>[2x]MVRQHAGPRDRSEIVTTSTGTNGRHTVAGPGSAGPVGYSLPLSPTGESAMLTPPPWHFSGEVVMVDYRVDPDAARRFLPPGLEPGADPGA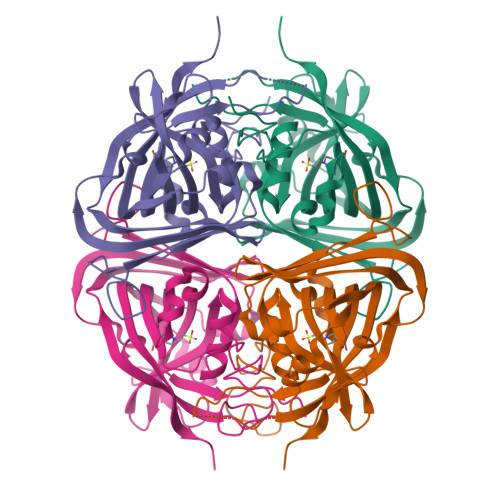AAAVFATWQWCSQDGAELTDPGRCQFGEFLILLSCEFEGRPMARCPYAWVDQAVPMMRGWVQGMPKQFGVIHQSRPVTVGKAGSRLAPGGRFDGALSVHGRRVVEASVTVDRSTDQPPALHDVPLAHTLVFPEWVPSGGGPRPRLVASEVSDVEFSPIWTGSGDLTFFDGLGDDFGALAPLEVGSGHVFSYGETLHGGRLLSDYSVSERHQP> MNREPLPIVVLISGNGTNLQAIIGAIQKGLAIEIRAVISNRADAYGLKRAQQADIPTHIIPHEEFPSRTDFESTLQKTIDHYDPKLIVLAGFMRKLGKAFVSHYSGRMINIHPSLLPKYTGLNTHER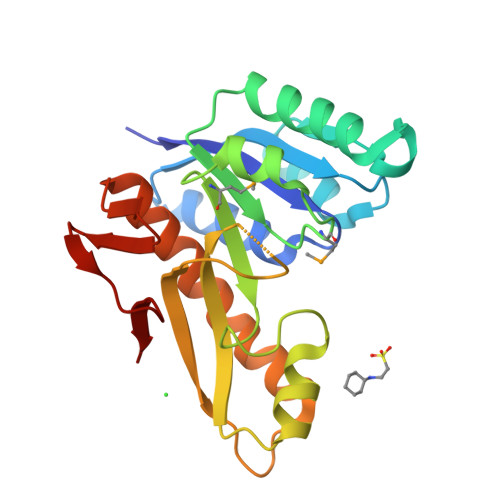ALAAGETEHGVSVHYVTEDLDAGPLICQARLSITPQDTPETLKTRVHALEHIIYPEVLSWFAAGRLNYHNNQVFLDGKPLAKSGHAFP2,6-bis(fluoranyl)-4-[4-(4-morpholin-4-ylphenyl)pyridin-3-yl]phenol | C21 H18 F2 N2 O2 | 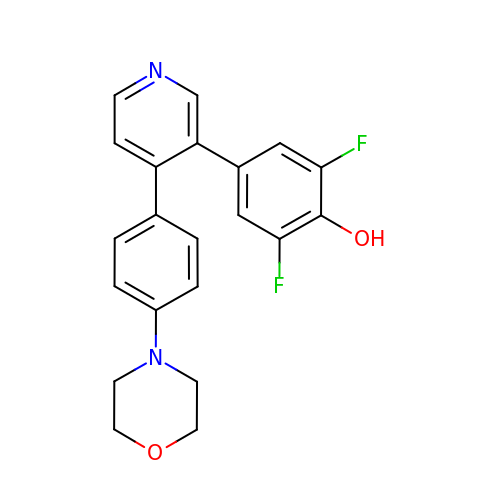YUYJEQHNWKQNBT-UHFFFAOYSA-N>HGFVSGIVADGKYYGGYLVNQYPYMSNPPDTIAWSTTATDLGFVDGTGYQSPDIICHRDAKNGKLTATVAAGSQIEFQWTTWPESHHGPLITYLAPCNGDCATVDKTTLKFVKIAAQGLIDGSNPPGVWADDEMIANNNTATVTIPASYAPGNYVLRHEIIALHSAGNLNGAQNYPQCFNIQITGG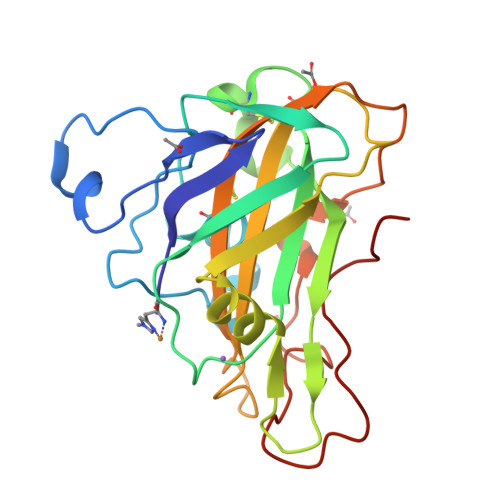GSAQGSGTAGTSLYKNTDPGIKFDIYSDLSGGYPIPGPALFNA[2x]>[2x]MADKELKFLVVDDFSTMRRIVRNLLKELGFNNVEEAEDGVDALNKLQAGGYGFVISDWRMPNMDGLELLKTIRADGAMSALPVLMVTAEAKKENIIAAAQAGASGYVVKPFTAATLEE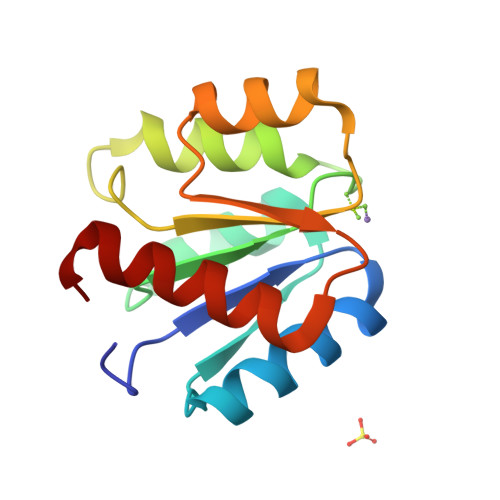KLNKIFEKLGM>MSFTVIIPARFASSRLPGKPLADIKGKPMIQHVFE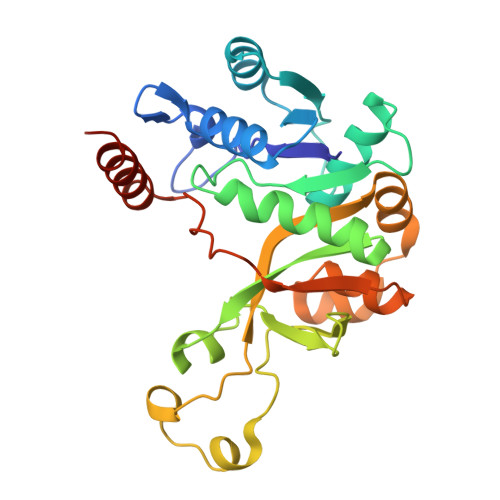KALQSGASRVIIATDNENVADVAKSFGAEVCMTSVNHNSGTERLAEVVEKLAIPDNEIIVNIQGDEPLIPPVIVRQVADNLAKFNVNMASLAVKIHDAEELFNPNAVKVLTDKDGYVLYFSRSVIPYDRDQFMNLQDVQKVQLSDAYLRHIGIYAYRAGFIKQYVQWAPTQLENLEKLEQLRVLYNGERIHVELAKEVPAVGVDTAEDLEKVRAILAANGSHHHHHH[2x]N-{[(4-chlorophenyl)carbonyl]carbamoyl}-beta-D-glucopyranosylamine | C14 H17 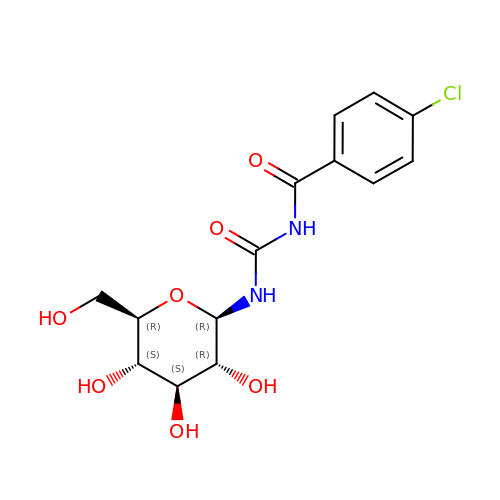Cl N2 O7 | YTUMHTAWGXUOIS-BZNQNGANSA-N> MPSTLEARA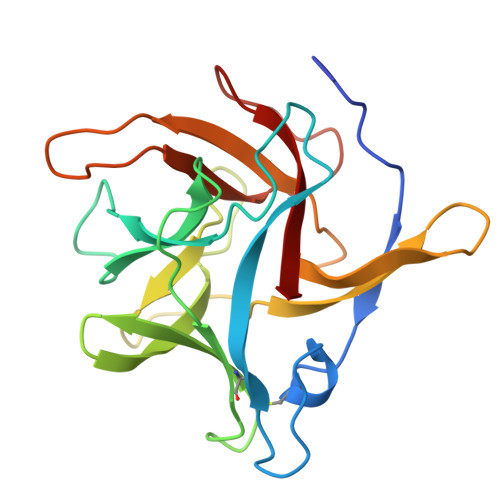LPQVSAVAKPRACSSYPTFDPATGEATEFIFYADSTEEPVAPFAGSVVGKLANPNLAIARIGIAVRGDLAKVVTKCFPDGGEEGLRTRTHGDWRRLTLAGGEDENIILIGQGPVAHRPLTPHDHFFANGTQQPGVFMGDNGSTTWAFSRKDASASEPFDQYEIRLLKSADSPLRNGEFRGFVRAA>GPHMTGLAAISDALAADLAGLSFSSPVAHVYNPLLYAREPHVAYLSRFGSPPKEVLFVGMDPGPWGMAQTGVPFGEVAVVTEWLGINGTVTRPAGEHPKKRVDGFACRRSEVSGRRLWGFIRERFGTPERFFARFFVANYCPLLFLTAEGGNITPDKLRRGE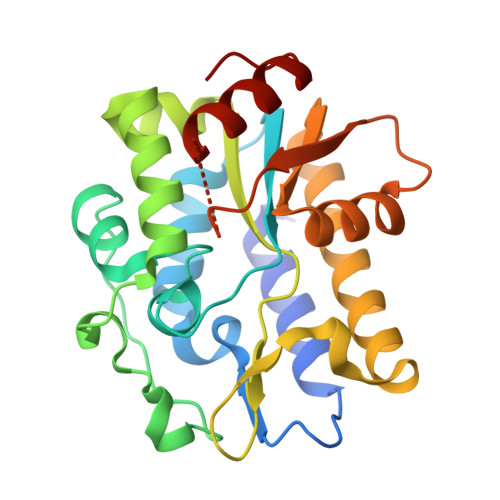QEPLFAACDLALRRTVVLLRPRVVIGVGAFAEARCHEALEGFDVEVGRIIHPSPASPAANRDWAGTALRQLAELGVDF[2x]>[2x]LRDLVCYCRTRGCKRRERMNGTCR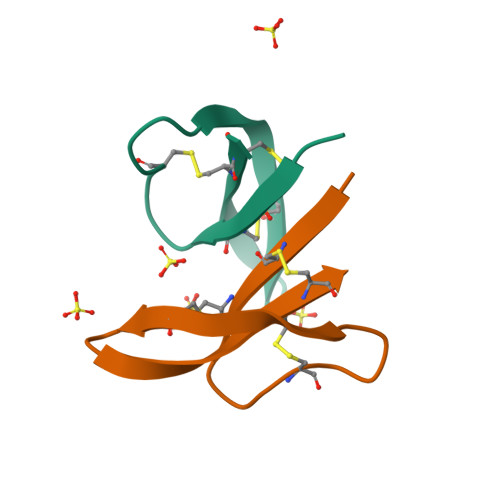KGHLMHTLCCR>GAMGSGVLPRPCRVLVLLNPRGGKGKALQLFRSHVQPLLAEAEISFTLMLTERRNHARELVRSEELGRWDALVVMSGDGLMHEVVNGLMERPDWETAIQKPLCSLPAGSGNALAASLNHYAGYEQVTNEDLLTNCTLLLCRRLLSPMNLLSLHTASGLRLFSVLSLAWGFIADVDLESEKYRRLGEMRFTLGTFLRLAALRTYRGRLAYLPVGRVGSKTPASPVVVQQGPVDAHLVPLEEPVPSHWTVVPDEDFVLVLALLHSHLGSEMFAAPMGRCAAGVMHLFYVRAGVSRAMLLRLFLAMEKGRHMEYECPYLVYVPVVAFRLEPKDGKGVFAV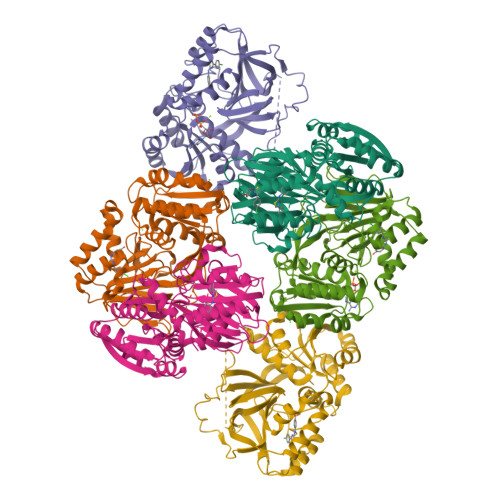DGELMVSEAVQGQVHPNYFWMVSG[6x]> MRRLEEDAVRVAYAGLRRKEAFKALAEKLGFTPLLFPVQATEKVPVPEYRDQVRALAQGVDLFLATTGVGVRDLMEAGKALGLDLEGPLAKAFRLARGAKAARALKEA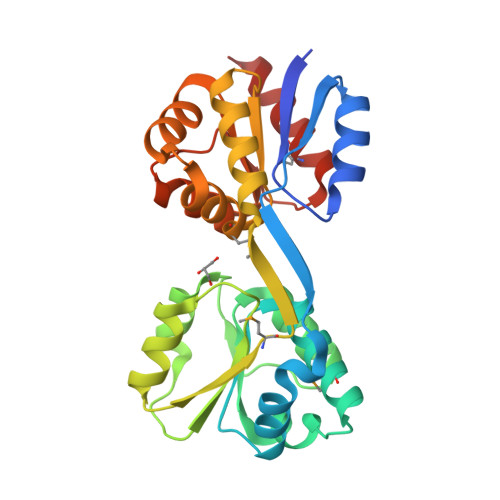GLPPHAVGDGTSKSLLPLLPQGRGVAALQLYGKPLPLLENALAERGYRVLPLMPYRHLPDPEGILRLEEALLRGEVDALAFVAAMQVEFLFEGAKDPKALREALNTRVKALAVGRVTADALREWGVKPFYVDETERLGSMLQGFKRALQKEVA>[4x]MAPVLSKDVADIESILALNPRTQSHAALHSTLAKKLDKKHWKRNPDKNCFHCEKLENNFDDIKHTTLGERGALREAMRCLKCADAPCQKSCPTHLDI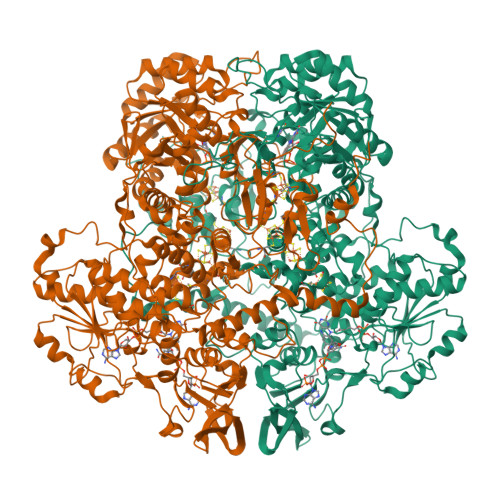KSFITSISNKNYYGAAKMIFSDNPLGLTCGMVCPTSDLCVGGCNLYATEEGSINIGGLQQFASEVFKAMNIPQIRNPCLPSQEKMPEAYSAKIALLGAGPASISCASFLARLGYSDITIFEKQEYVGGLSTSEIPQFRLPYDVVNFEIELMKDLGVKIICGKSLSENEITLNTLKEEGYKAAFIGIGLPEPKTDDIFQGLTQDQGFYTSKDFLPLVAKSSKAGMCACHSPLPSIRGAVIVLGAGDTAFDCATSALRCGARRVFLVFRKGFVNIRAVPEEVELAKEEKCEFLPFLSPRKVIVKGGRIVAVQFVRTEQDETGKWNEDEDQIVHLKADVVISAFGSVLRDPKVKEALSPIKFNRWDLPEVDPETMQTSEPWVFAGGDIVGMANTTVESVNDGKQASWYIHKYIQAQYGASVSAKPELPLFYTPVDLVDISVEMAGLKFINPFGLASAAPTTSSSMIRRAFEAGWGFALTKTFSLDKDIVTNVSPRIVRGTTSGPMYGPGQSSFLNIELISEKTAAYWCQSVTELKADFPDNIVIASIMCSYNKNDWMELSRKAEASGADALELNLSAPHGMGERGMGLACGQDPELVRNICRWVRQAVQIPFFAKLTPNVTDIVSIARAAKEGGADGVTATNTVSGLMGLKADGTPWPAVGAGKRTTYGGVSGTAIRPIALRAVTTIARALPGFPILATGGIDSAESGLQFLHSGASVLQVCSAVQNQDFTVIQDYCTGLKALLYLKSIEELQGWDGQSPGTESHQKGKPVPRIAELMGKKLPNFGPYLEQRKKIIAEEKMRLKEQNAAFPPLERKPFIPKKPIPAIKDVIGKALQYLGTFGELSNIEQVVAVIDEEMCINCGKCYMTCNDSGYQAIQFDPETHLPTVTDTCTGCTLCLSVCPIIDCIRMVSRTTPYEPKRGLPLAVNPVC>[2x]AFEDRDPTQFEERHLKFLQQLGKGNFGSVEMCRYDPLQDNTGEVVAVKKLQHSTEEHLRDFEREIEILKSLQHDNIVKYKGV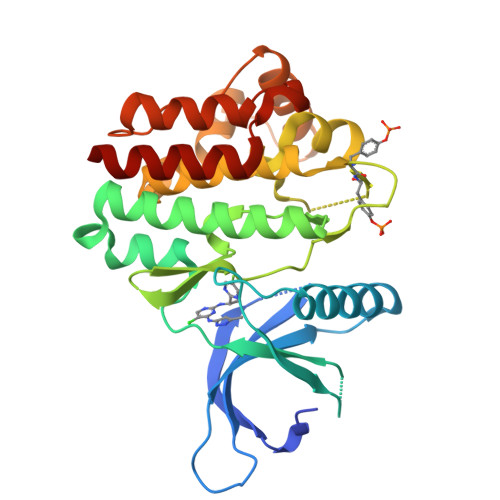CYSAGRRNLKLIMEYLPYGSLRDYLQAHAERIDHIKLLQYTSQICKGMEYLGTKRYIHRDLATRNILVENENRVKIGDFGLTKVLPQDKEYYKVKEPGESPIFWYAPESLTESKFSVASDVWSFGVVLYELFTYIEKSKSPPAEFMRMIGNDKQGQMIVFHLIELLKNNGRLPRPDGCPDEIYMIMTECWNNNVNQRPSFRDLALRVDQIRDNMAG As an E2, Cdc34 is the central player in a cascade of enzymes that includes an E1 ubiquitin activating enzyme, Uba1, and a large family of Skp-Cullin-F-box (SCF) E3 ubiquitin ligases that function in tandem to assemble Lys48-linked Ub chains on proteins to target them for proteasomal degradation. Uba1 is a multidomain enzyme that serves as the gatekeeper of the Ub conjugation cascade by activating Ub in a two-step process involving adenylation and thioester bond formation followed by transfer of Ub to E2s in a process termed E1-E2 thioester transfer or transthiolation. Additionally, Cdc34 contains unique structural features that are crucial for efficient polyUb chain extension through poorly understood mechanisms, including an acidic loop insertion proximal to the active site and a long C-terminal extension. To better understand the molecular bases of Cdc34 activities, we here determine crystal structures of Cdc34 alone and in complex with Uba1, as well as a Cdc34~Ub mimetic that represents the product of E1-E2 thioester transfer.

To investigate potential Cdc34 conformational changes that accompany Uba1 binding, a 1.7 Å structure of ScCdc34Δdist alone, Cdc34apo, was determined. Comparison of Cdc34apo and Cdc34E1-bound reveals two conformational changes that accompany Uba1 binding, both within E1-interacting regions. When bound to Uba1, this extended region of hA melts but remains ordered and projects away from the helix. The second conformational change occurs on the opposite side of the E2, where hC of Cdc34apo (hCapo) is extended N-terminally by one residue and sits at a different angle compared to hCE1-bound. Modeling Cdc34apo onto the Uba1–Cdc34 complex reveals a mechanistic role for Cdc34 conformational changes that accompany Uba1 binding (middle). Second, the extension and altered angle of hCapo positions Val143 such that it clashes with the SCCH, whereas Cdc34E1-bound Val143 is shifted away from the SCCH and makes productive contacts with Uba1 Asn694 and Phe695 (and 5b, right). Our Cdc34apo and Uba1-Cdc34 structures reveal combinatorial Uba1 recognition of Cdc34 involving a distinct Cdc34/UFD interface and conformational changes in Cdc34 that accompany Uba1 binding.

> GAMASRKSTASSLLLRQYRELTDPKKAIPSFHIELEDDSNIFTWNIGVMVLNEDSIYHGGFFKAQMRFPEDFPFSPPQFRFTPAIYHPNVYRDGRLCISILHQSGDPMTDEPDAETWSPVQTVESVLISIVSLLEDPNINSPANVDAAVDYRKNPEQYKQRVKMEVERSKQDIPKGFIMPTSESAYISQSKLDEPES PDE6D has been shown to bind farnesylated RAS proteins and facilitate their trafficking and plasma membrane (PM) localization. PDE6D has been reported to chaperone NRAS, HRAS, and KRAS4B but not KRAS4A. We determined the direct target of DW0254 to be PDE6D, a chaperone protein that facilitates cytoplasmic trafficking of farnesylated molecules, including RAS, as a target for this compound, thus linking RAS transport with RAC GTPase activation in leukemic cells. The results presented here provide evidence of the importance of PDE6D in sustaining downstream RAS signaling and cell survival in a large panel of acute leukemia cell lines.

E Docking results in wild type apo structure of PDE6D and R48delV49del mutant; Root mean square deviation (RMSD) with respect to 3D coordinates of the ligands in the superposed X-ray complex of the wild type protein are reported. In addition, in silico docking of DW0254 to R48del V49del PDE6D confirmed an accentuated increase in the root mean square deviation (RMSD) in contrast with Deltarasin’s RMSD that was only marginally affected, strongly suggesting DW0254 would be unlikely to bind PDE6D in the event of deletion of these two residues. Interestingly, the combination of DW0254 and Deltarasin had a significant synergistic effect suggesting that these compounds might be targeting singular conformations of PDE6D with different efficiencies. Indeed, large conformational changes in PDE6D to facilitate the binding of farnesylated RAS proteins deeper within the hydrophobic pocket have been previously described.

> MGSHHHHHHGSENLYFQSAKDERAREILRGFKLNWMNLRDAETGKILWQGTEDLSVPGVEHEARVPKKILKCKAVSRELNFSSTEQMEKFRLEQKVYFKGQCLEEWFFEFGFVIPNSTNTWQSLIEAAPESQMMPASVLTGNVIIETKFFDDDLLVSTSRVRLFYV N-cyclopropyl-5-methyl-N-(propan-2-yl)-1,2-oxazole-3-carboxamide 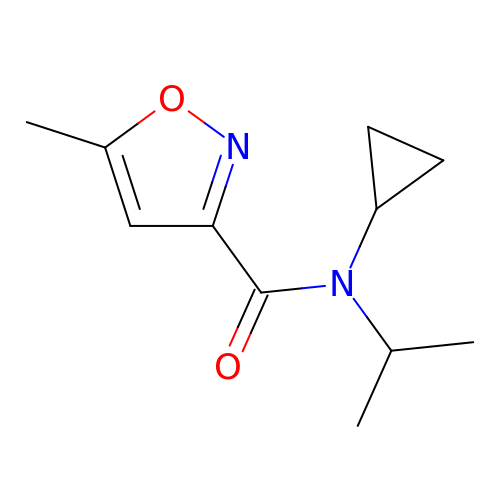| C11 H16 N2 O2 | KOQGLXMVOJEOLV-UHFFFAOYSA-N>[4x]GSAAASSVDTSQEFQNNLKNAIGNLPFQYVNGI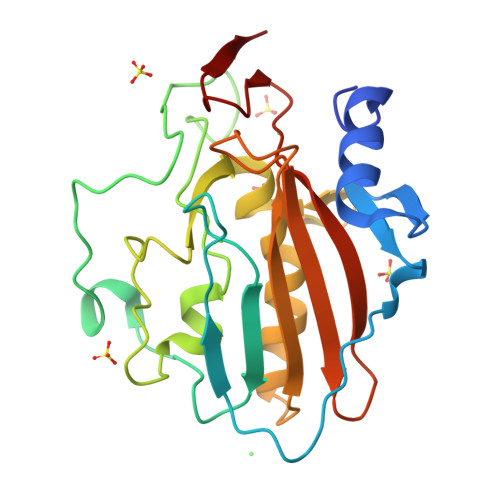YELNNNQTNLNADVNVKAYVQNTIDNQQRPSTANAMLDRTIRQYQNRRDTTLPDANWKPLGWHQVATNDHYGHAVDKGALIAYALAGNFKGWDASVSNPQNVVTQTAHSNQSNQKINRGQNYYESLVRKAVDQNKRVRYRVTPLYRNDTDLVPFAMHLEAKSQDGTLEFNVAIPNTQASYTMDYATGEITLN> MVECITPEAIFIGANKQTQVSDIHKVKKIVAFGAGKTIALWDPIEPNNKGVYATLKGHEAEVTCVRFVPDSDFMVSASEDHHVKIWKFTDYSHLQCIQTIQHYSKTIVALSALPSLISVGCADGTISIWRQNIQNDEFGLAHEFTIKKGFFYPLCLSLSKVEEKKYLLAIGGTNVNVFIASFILSDSGIEKCRVVAELEGHEDWVKSLAFRHQETPGDYLLCSGSQDRYIRLWRIRINDLIDDSEEDSKKLTLLSNKQYKFQIDDELRVGINFEALIMGHDDWISSLQWHESRLQLLAATADTSLMVWEPDETSGIWVCSLRLGEMSSKGASTATGSSGGFWSCLWFTHERMDFFLTNGKTGSWRMWATKDNIICDQRLGISGATKDVTDIAWSPSGEYLLATSLDQTTRLFAPWIYDASGRKREIATWHEFSRPQIHGYDMICVETVTDTRFVSGGDEKILRSFDLPKGVAGMLQKFVGIQFE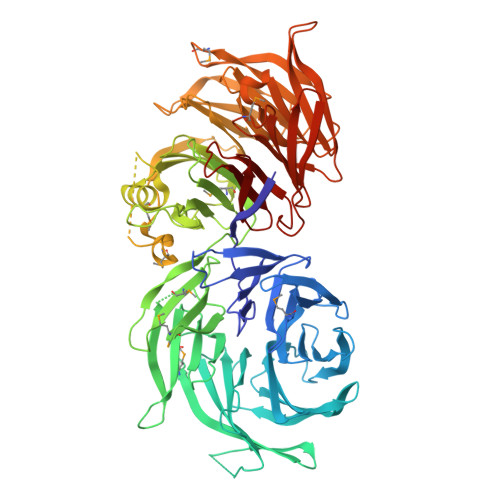EKSEMPDSATVPVLGLSNKAGEDDANEDDEEEEGGNKETPDITDPLSLLECPPMEDQLQRHLLWPEVEKLYGHGFEITCLDISPDQKLIASACRSNNVQNAVIRIFSTENWLEIKPALPFHSLTITRLKFSKDGKFLLSVCRDRKWALWERNMEDNTFELRFKNEKPHTRIIWDADWAPLEFGNVFVTASRDKTVKVWRHQKEPADDYVLEASIKHTKAVTAISIHDSMIREKILISVGLENGEIYLYSYTLGKFELITQLNEDITPADKITRLRWSHLKRNGKLFLGVGSSDLSTRIYSLAYE> MSEFAMVFPGQGSQDLGMLADLATAFPVVEQTFAEASDVLGYDLWALVQQGPEEELNKTWQTQPALLAASVAIWRVWQEKGGKAPSLMAGHSLGEYSALVCAGVIDFKQAIRLVELRGKLMQEAVPEGTGAMYVIIGLDNESIDRACKEVAQGQIVSPVNFNSPGQVVIAGEKEAVERAGDACKAAGAKRALPLAVSVPSHCALMKPAADKLAVVLEGIEFGYPQFPVVNNVDVKIEQSAEAIRHALVRQLYNPVRWTETVEFITEQGVG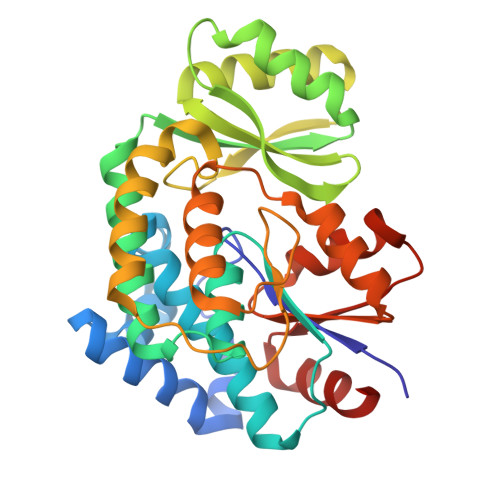QLLEIGPGRVLTGLTKRIVNTLSAAAVNDTASLITALENN> MGSSHHHHHHSSGENLYFQG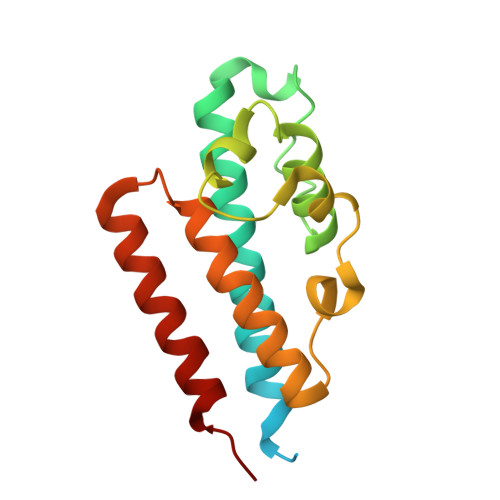SYAHIPGIETPPLQFDKVSQNVFEQVKETIFFAIDHTLRKEYGEDIGFIDYNPDKLTTIENASNYIYLFWVSVFSELFTCSKIKKNEWKSLPTVLKSKPTNLNDLRTFEQFWETVLHFLFSKFTNEEKQSLEKQIHEWKTSINAIST> GSSDDEDSVRYLLYMAELRYEQGNPEKAKKILEMAEFI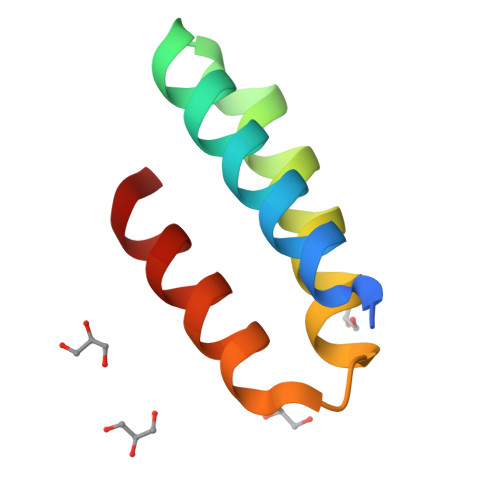AKRNNNEELERLVREVKKRL>SNAMNSEQADILDLLSGHTDDTTIERLAFECLLTNMTDDRVVSLMNILGWQGDFNCFAIGGVPSASLASTSLAIRKAVRDLGGEHVVIGTYGTFLLALACQMGAVTPEVTCTAVMPAFSEDEPLYLSPVRSGVAGASHALRETMFSLQAAPALSTPSRPLRADELLPERALLGDDYAREELYRNVYQVLRGENPDDPTYLTVSTFLKYGSSLENTAKELNV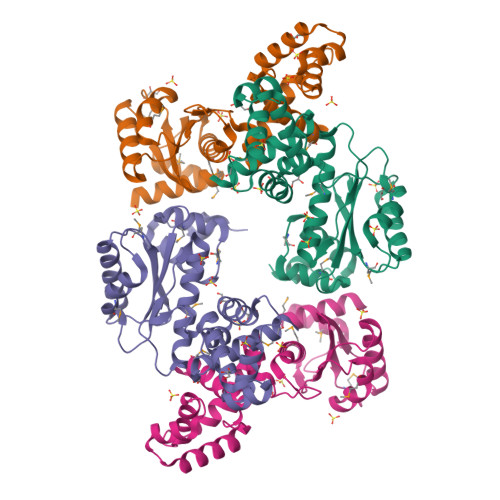HPNTVRYRLKRAAETTGWDATDPRDAYVLTTALAIGRMRDR[4x]>SHMLRPVETPTREIKKLDGLWAFSLD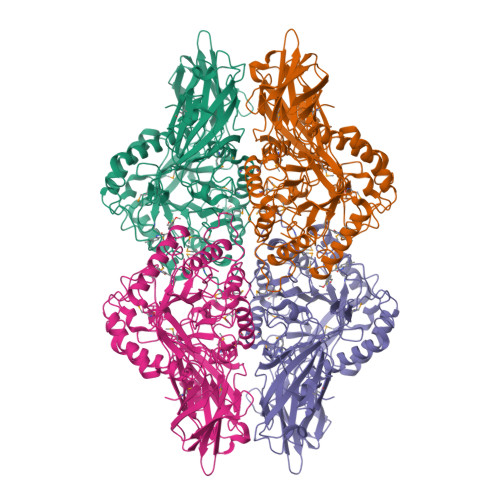RENCGIDQRWWESALQESRAIAVPGSFNDQFADADIRNYAGNVWYQREVFIPKGWAGQRIVLRFDAVTHYGKVWVNNQEVMEHQGGYTPFEADVTPYVIAGKSVRITVCVNNELNWQTIPPGMVITDENGKKKQSYFHDFFNYAGIHRSVMLYTTPNTWVDDITVVTHVAQDCNHASVDWQVVANGDVSVELRDADQQVVATGQGTSGTLQVVNPHLWQPGEGYLYELCVTAKSQTECDIYPLRVGIRSVAVKGEQFLINHKPFYFTGFGRHEDADLRGKGFDNVLMVHDHALMDWIGANSYRTSHYPYAEEMLDWADEHGIVVIDETAAVGFNLSLGIGFEAGNKPKELYSEEAVNGETQQAHLQAIKELIARDKNHPSVVMWSIANEPDTRPQGAREYFAPLAEATRKLDPTRPITCVNVMFCDAHTDTISDLFDVLCLNRYYGWYVQSGDLETAEKVLEKELLAWQEKLHQPIIITEYGVDTLAGLHSMYTDMWSEEYQCAWLDMYHRVFDRVSAVVGEQVWNFADFATSQGILRVGGNKKGIFTRDRKPKSAAFLLQKRWTGMNFGEKPQQGGKQ[2x]>[40x]AEGDDPAKAAFNSLQAS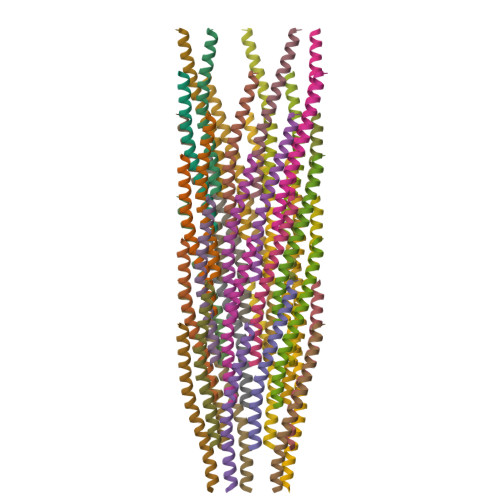ATEYIGYAWAMVVVIVGATIGIKLFKKFTSKAS> MNNFIPQPQGLLRFLNTLDTDLTSSHMNLLDEEVSFVSKFYTPQLQLSELAKKVLTNIKTDDIPVLEREFNDNTIIHK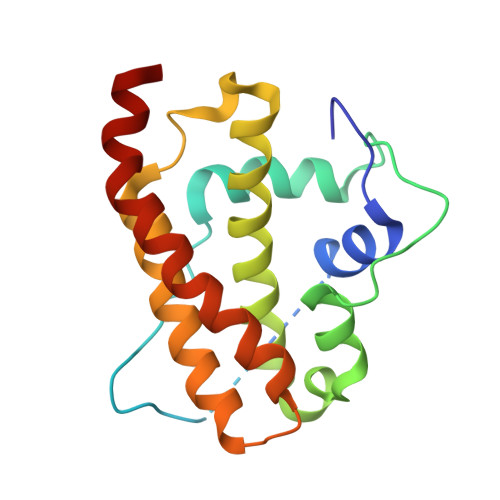ANDTLLKVQAPRMYMILQSIVLEAYAIVNCFVENPSSLKYLTEEDVSITRENLNYVADYLGNYDDYNSVVLDLRDLDLCFSAIELQLPLIKKEANV N,O-DIDANSYL-L-TYROSINE | C33 H33 N3 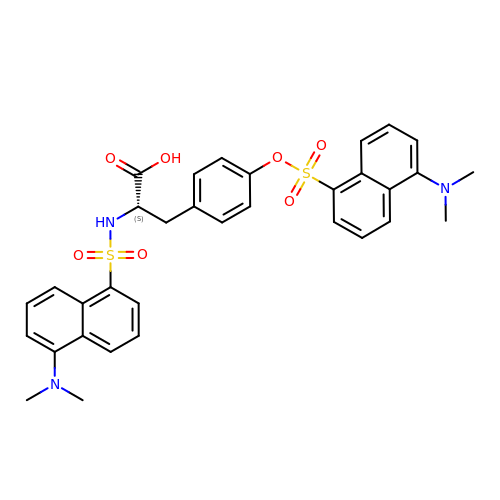O7 S2 | LUBOPDUYHWABFG-NDEPHWFRSA-N>[2x]MVLYFIGLGLYDERDITVKGLEIAKKCDYVFAEFYTSLMAGTTLGRIQKLIGKEIRVLSREDVELNFENIVLPLAKENDVAFLTPGDPLVATTHAELRIRAKRAGVESYVIHAPSIYSAVGITGLHIYKFGKSATVAYPEGNWFPTSYYDVIKENAERGLHTLLFLDIKAEKRMYMTANEAMELLLKVEDMKKGGVFTDDTLVVVL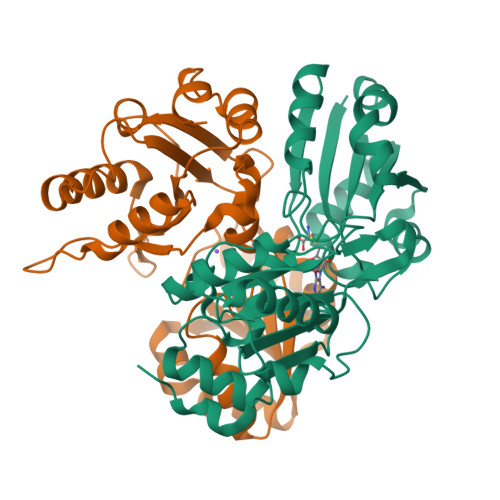ARAGSLNPTIRAGYVKDLIREDFGDPPHILIVPGKLHIVEAEYLVEIAGAPREMLRVNV> MLTYGAPFNFPRWIDEHAHLLKPPVGNRQVWQDSDFIVTVVGGPNHRTDYHDDPLEEFFYQLRGNAYLNLWVDGRRERADLKEGDIFLLPPHVRHSPQRPEAGSACLVIERQRPAGMLDGFEWYCDACGHLVHRVEVQLKSIVTDLPPLFESFYASEDKRRCPHCG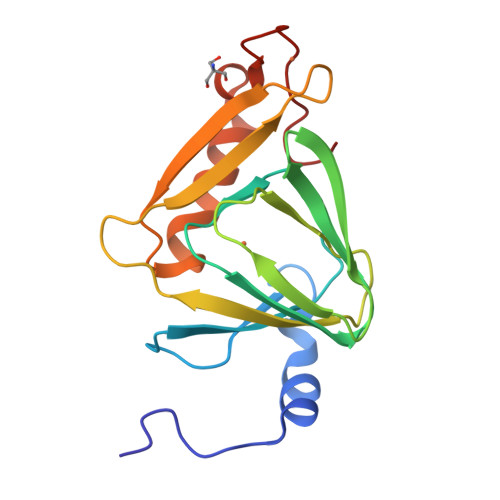QVHPGRAA>MTINYHE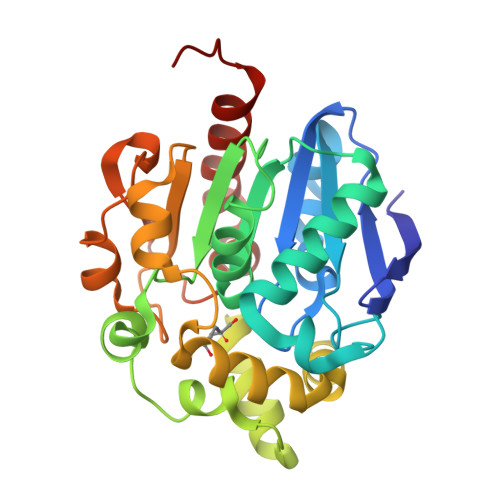LETSHGRIAVRESEGEGAPLLMIHGNSSSGAIFAPQLEGEIGKKWRVIAPDLPGHGKSTDAIDPDRSYSMEGYADAMTEVMQQLGIADAVVFGWSLGGHIGIEMIARYPEMRGLMITGTPPVAREEVGQGFKSGPDMALAGQEIFSERDVESYARSTCGEPFEASLLDIVARTDGRARRIMFEKFGSGTGGNQRDIVAEAQLPIAVVNGRDEPFVELDFVSKVKFGNLWEGKTHVIDNAGHAPFREAPAEFDAYLARFIRDCTQLEHHHHHH[2x]> MTHGAVKTYGIRLRVWGDYACFTRPEMKVERVSYDVMPPSAARGILEAIHWKPAIRWIVDRIHVLRPIVFDNVRRNEVSSKIPKPNPATAMRDRKPLYFLVDDGSNRQQRAATLLRNVDYVIEAHFELTDKAGAEDNAGKHLDIFRRRARAGQSFQQPCLGCREFPASFELLEGDVPLSCYAGEKRDLGYMLLDIDFERDMTPLFFKAVMEDGVITPPSRTSPEVRA;>MTAIANRYEFVLLFDVENGNPNGDPDAGNMPRIDPETGHGLVTDVCLKRKIRNHVALTKEGAERFNIYIQEKAILNETHERAYTACDLKPEPKKLPKKVEDAKRVTDWMCTNFYDIRTFGAVMTTEVNCGQVRGPVQMAFARSVEPVVPQEVSITRMAVTTKAEAEKQQGDNRTMGRKHIVPYGLYVAHGFISAPLAEKTGFSDEDLTLFWDALVNMFEHDRSAARGLMSSRKLIVFKHQNRLGNAPAHKLFDLVKVSRAEGSSGPARSFADYAVTVGQAPEGVEVKEML[7x];> MILQALHGYYQRMSADPDAGMPPYGTSMENISFALVLDAKGTLRGIEDLREQEGKKLRPRKMLVPIAEKKGNGIKPNFLWENTSYILGVDAKGKQERTDKCHAAFIAHIKAYCDTADQDLAAVLQFLEHGEKDLSAFPVSEEVIGSNIVFRIEGEPGFVHERPAARQAWANCLNRREQGLCGQCLITGERQKPIAQLHPSIKGGRDGVRGAQAVASIVSFNNTAFESYGKEQSINAPVSQEAAFSYVTALNYLLNPSNRQKVTIADATVVFWAERSSPAEDIFAGMFDPPSTTAKPESSNGTPPEDSEEGSQPDTARDDPHAAARMHDLLVAIRSGKRATDIMPDMDESVRFHVLGLSPNAARLSVRFWEVDTVGHMLDKVGRHYRELEIIPQFNNEQEFPSLSTLLRQTAVLNKTENISPVLAGGLFRAMLTGGPYPQSLLPAVLG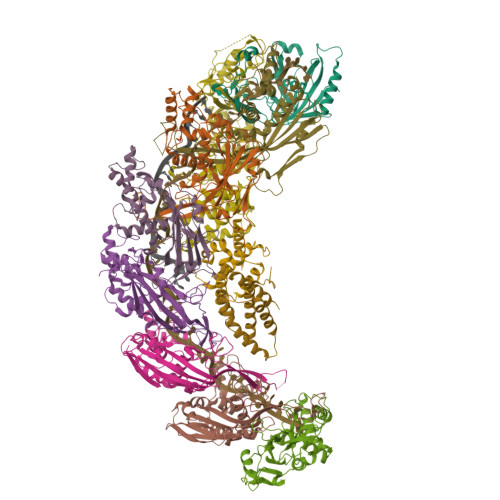RIRAEHARPEDKSRYRLEVVTYYRAALIKAYLIRNRKLEVPVSLDPARTDRPYLLGRLFAVLEKAQEDAVPGANATIKDRYLASASANPGQVFHMLLKNASNHTAKLRKDPERKGSAIHYEIMMQEIIDNISDFPVTMSSDEQGLFMIGYYHQRKALFTKKNKEN;>[2x]VSLDPARTDRPYLLGRLFAVLEKAQEDAVPGANATIKDRYLASASANPGQVFHMLLKNASNHTAKLRKDPERKGSAIHYEIMMQEIIDNISDFPVTMSSDEQGLFMIGYYHQRKALFTKKNKEN> DNRLGL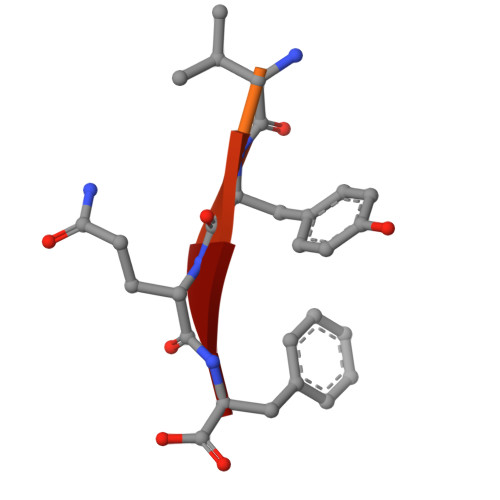VYQF METHYL-3-(4'-N-OXOPYRIDYLPHENOYL)-3-METHYL-2-(M-AMIDINOBENZYL)-PROPIONATE 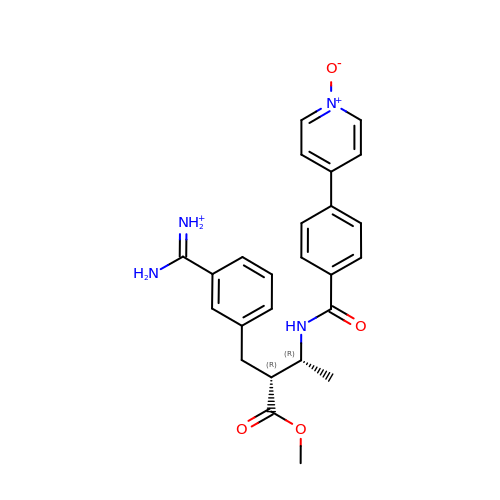| C25 H27 N4 O4 | PFGVNLZDWRZPJW-OPAMFIHVSA-O>[4x]SMAKNRRDRNSWGGFSEKTYEWSSEEEEPVKKAGPVQVLIVKDDHSFELDETALNRILLSEAVRDKEVVAVSVAGAFRKGKSFLMDFMLRYMYNQESVDWVGDYNEPLTGFSWRGGSERETTGIQIWSEIFLINKPDGKKVAVLLMDTQGTFDSQSTLRDSATVFALSTMISSIQVYNLSQNVQEDDLQHLQLFTEYGRLAMEETFLKPFQSLIFLVRDWSFPYEFSYGADGGAKFLEKRLKVSGNQHE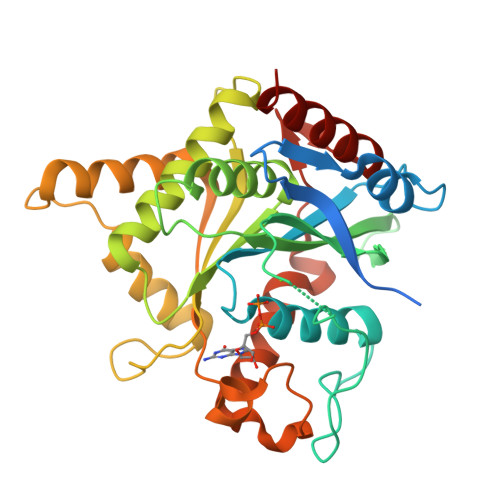ELQNVRKHIHSCFTNISCFLLPHPGLKVATNPNFDGKLKEIDDEFIKNLKILIPWLLSPESLDIKEINGNKITCRGLVEYFKAYIKIYQGE>[2x]MWVKILSVVGARPQFIKAAAVSRVLRASPGVREVLVHTGQHYDDNMSQVFFEELEIPDPDYHLGIGGGTHGQNTGRMLEAIEGVLLKEKPDWVLVYGNTDSTLAGALAAVKLHIPVAHVEAGLRSFNRRMPEEINRILTDHASDLLFAPTETAVQNLLREGIPENRIHLVGDVMYDAALHYGAKAERKSRILERLGLQAKGYVLA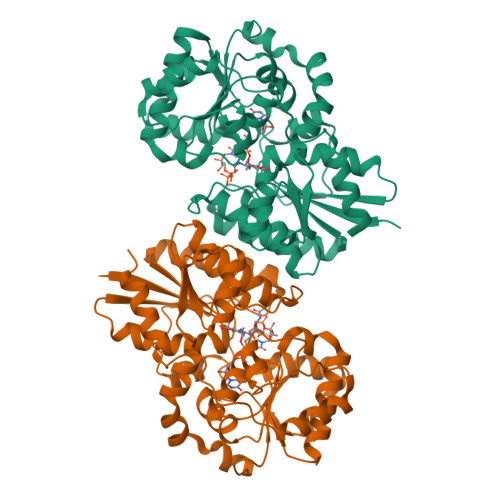TIHRAENTDDQERLRVILEALAEVHQEVPVVFPVHPRTRKRAEAFGLGSYLEKVVALEPVGYLDMVMLEKNARLIVTDSGGVQKEAYFYRVPCVTVREETEWVELLKAEWNYLAAPQNAKDLALTILHRMRTKGVEIDLYGDGRASQKISDFLRKVGIRTLEHHHHHH>MMSETAPLPSASSALEDKAASAPVVGIIMGSQSDWETMRHADALLTELEIPHETLIVAAHRTPDRLADYARTAAERGLNVIIAGAGGAAHLPGMCA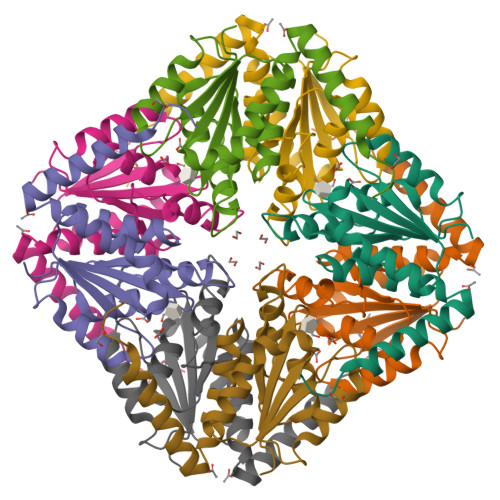AWTRLPVLGVPVESRALKGMDSLLSIVQMPGGVPVGTLAIGASGAKNAALLAASILALYNPALAARLETWRALQTASVPNSPITEDK[2x]>[2x]MEKDTKQVDI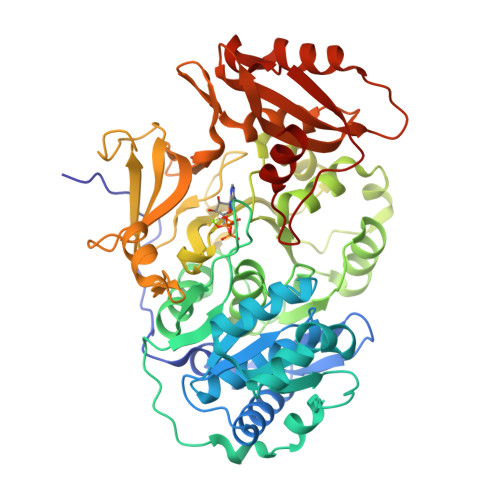IFRSKLPDIYIPNHLPLHSYCFENISEFSSRPCLINGANKQIYTYADVELNSRKVAAGLHKQGIQPKDTIMILLPNSPEFVFAFIGASYLGAISTMANPLFTPAEVVKQAKASSAKIIVTQACHVNKVKDYAFENDVKIICIDSAPEGCLHFSVLTQANEHDIPEVEIQPDDVVALPYSSGTTGLPKGVMLTHKGLVTSVAQQVDGENPNLYIHSEDVMLCVLPLFHIYSLNSVLLCGLRVGAAILIMQKFDIVSFLELIQRYKVTIGPFVPPIVLAIAKSPMVDDYDLSSVRTVMSGAAPLGKELEDTVRAKFPNAKLGQGYGMTEAGPVLAMCLAFAKEPFEIKSGACGTVVRNAEMKIVDPKTGNSLPRNQSGEICIRGDQIMKGYLNDPEATARTIDKEGWLYTGDIGYIDDDDELFIVDRLKELIKYKGFQVAPAELEALLLNHPNISDAAVVPMKDEQAGEVPVAFVVRSNGSTITEDEVKDFISKQVIFYKRIKRVFFVDAIPKSPSGKILRKDLRAKLAAGLPN> KVSGTVCLSALPPEATKTLNLIASKGPFPYSQDGVVFQNRKSVLPTQSYGYYHEYTVITPGARTRGTRRIITGKATQEDYYTGDHYAT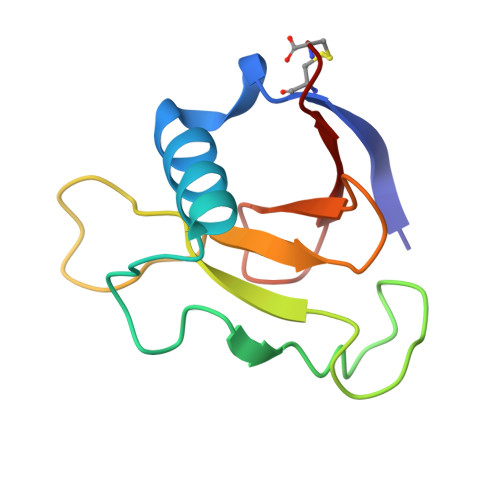FSLIDQTC>[6x]MQNGYTYED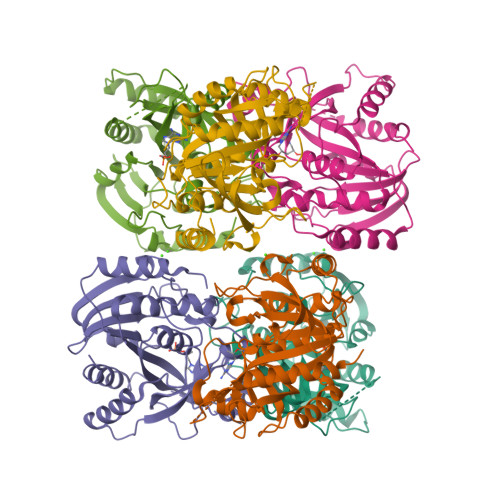YQDTAKWLLSHTEQRPQVAVICGSGLGGLVNKLTQAQTFDYSEIPNFPESTVPGHAGRLVFGILNGRACVMMQGRFHMYEGYPFWKVTFPVRVFRLLGVETLVVTNAAGGLNPNFEVGDIMLIRDHINLPGFSGQNPLRGPNEERFGVRFPAMSDAYDRDMRQKAHSTWKQMGEQRELQEGTYVMLGGPNFETVAECRLLRNLGADAVGMSTVPEVIVARHCGLRVFGFSLITNKVIMDYESQGKANHEEVLEAGKQAAQKLEQFVSLLMASIPVSGHTG>[2x]GAMDISGGNTSRQPQKKSNQNIQVYVRVRPLNSRERCIRSAEVVDVVGPREVVTRHTLD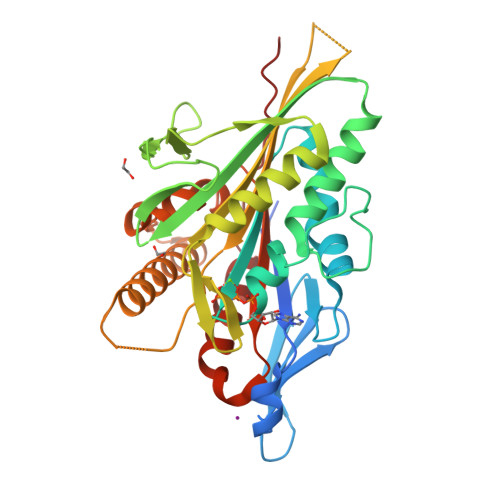SKLTKKFTFDRSFGPESKQCDVYSVVVSPLIEEVLNGYNCTVFAYGQTGTGKTHTMVGNETAELKSSWEDDSDIGIIPRALSHLFDELRMMEVEYTMRISYLELYNEELCDLLSTDDTTKIRIFDDSTKKGSVIIQGLEEIPVHSKDDVYKLLEKGKERRKTATTLMNAQSSRSHTVFSIVVHIRENGIEGEDMLKIGKLNLVDLAGSENVSKAGNEKGIRVRETVNINQSLLTLGRVITALVDRAPHVPYRESKLTRLLQESLGGRTKTSIIATISPGHKDIEETLSTLEYAHRAKNIQNKPEVNQKLT>ANRTLIVTTILEEPYVMYRKSDKPLYGNDRFEGYCLDLLKELSNILGFIYDVKLVPDGKYGAQNDKGEWNGMVKELIDHRADLAVAPLTITYVREKVIDFSKPFMTLGISIL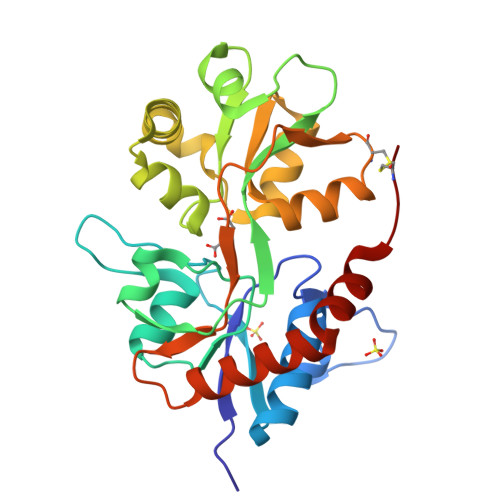YRKGTPIDSADDLAKQTKIEYGAVRDGSTMTFFKKSKISTYEKMWAFMSSRQQTALVRNSDEGIQRVLTTDYALLMESTSIEYVTQRNCNLTQIGGLIDSKGYGVGTPIGSPYRDKITIAILQLQEEGKLHMMKEKWWRGNGCP[2x]(2S)-2-[(3R)-3-(acetylamino)-3-(2-methylpropyl)-2-oxopyrrolidin-1-yl]-N-{(1R,2S)-3-(3,5-difluorophenyl)-1-hydroxy-1-[(2R,4R)-4-propoxypyrrolidin-2-yl]propan-2-yl}-4-phenylbutanamide 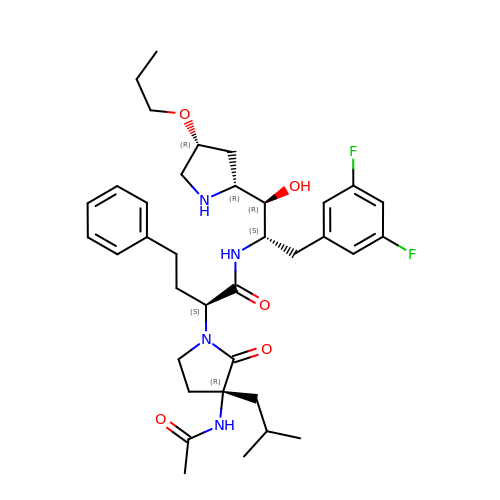| C36 H50 F2 N4 O5 | LPZOLMFQGUDKQH-ZXWXCOCLSA-N> MTKVTREEVEHI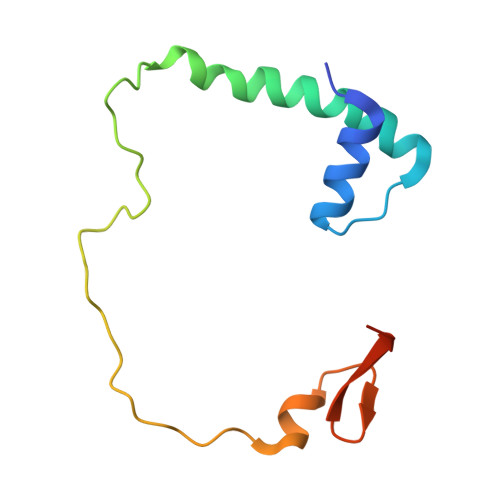ANLARLQISPEETEEMANTLESILDFAKQNDSADTEGVEPTYHVLDLQNVLREDKAIKGIPQELALKNAKETEDGQFKVPTIMNEEDA> GTTLSESFENGIPASWKTIDADGDGHGWKPGNAPGIAGYNSNGCVYSESFGLG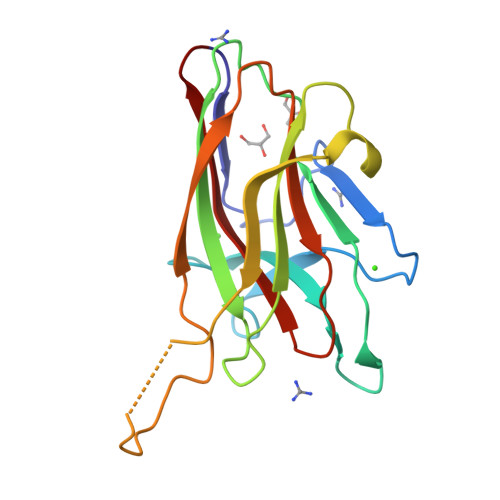GIGVLTPDNYLITPALDLPNGGKLTFWVCAQDANYASEHYAVYASSTGNDASNFTNALLEETITAKGVRSPKAIRGRIQGTWRQKTVDLPAGTKYVAFRHFQSTDMFYIDLDEVEIKANG In Bacillus subtilis, the RicA (YmcA), RicF (YlbF), and RicT (YaaT) proteins accelerate the phosphorylation of the transcription factor Spo0A, contributing to genetic competence, sporulation, and biofilm formation, and are also essential for the correct maturation of several protein-encoding and riboswitch RNAs. These proteins form a stable complex (RicAFT) that carries two [4Fe-4S]+2 clusters. We show here that the complex is a 1:1:1 heterotrimer, and we present the X-ray crystal structures of a RicAF heterotetramer and of a RicA dimer.

Each RicA protomer contains five α-helices, and dimerization is mediated by intermolecular contacts between helices α1, α2, and α5, forming a core antiparallel helical bundle that buries 1,887 Å2 of surface area. Outside this region, in each RicA protomer, helices α3 and α4 together form flaps that extend in a nearly orthogonal direction from the helical bundle core. The elution volume of RicA in SEC is consistent with it being a dimer (32.04 kDa). Despite the fact that RicA and RicF have only about 20% sequence identity, their monomeric structures as well as the structures of RicA and RicAF are nearly identical. In fact, superposition of RicA dimer and of RicAF revealed a root mean square deviation (RMSD) value for 166 aligned Cα of 0.982 Å. The most poorly aligned portions of these structures occurred in the α3-α4 flaps, suggesting that there may be some flexibility in the turns connecting α3 to α4 and α4 to α5. RicA can exist in complex with itself to form a homodimer or with RicF to form a tetramer. Using Pisa analysis, we have identified buried residues at the RicA-RicA and RicA-RicF interfaces, which we conservatively define as those with >20% buried surface area. Of 36 buried RicA residues in RicA-RicA, 28 are also buried in RicA-RicF. Because there is no evidence for a RicA tetramer, it would appear that the association of RicA with itself precludes tetramerization and, indeed, the tetramerization interface between RicAF dimers involves only RicA-RicF contacts (rather than RicA-RicA or RicF-RicF contacts).

> GPMTLYSKKDIVQQARNLAKMISETEEVDFFKRAEAQINENDKVSTIVNQIKALQKQAVNLKHYEKHEALKQVEAKIDALQEELEEIPVIQEFRDSQMEVNDLLQLVAHTISNQVTNEIITSTG>[2x]AACNGYVGLTFDDGPSGSTQSLLNALRQNGLRATMFNQGQYAAQNPSLVRAQVDAGMWVANHSYTHPHMTQLGQAQMDSEISRTQQAIAGAGGGTPKLFRPPYG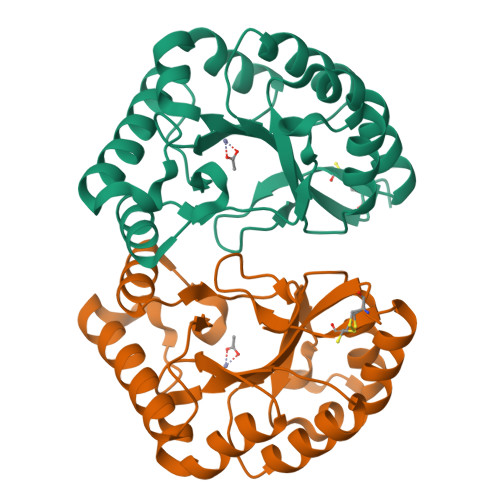ETNATLRSVEAKYGLTEVIWDVDSQDWNNASTDAIVQAVSRLGNGQVILMHDWPANTLAAIPRIAQTLAGKGLCSGMISPQTGRAVAPDGS> MALRAMRGIVNGAAPELPVPTSGPLAGSREQALAVSRNYLSQPRLTYKTVSGVNGPLVILDHVKFPRYAEIVHLTLPDGTKRSGQVLEVSGSKAVVQVFEGTSGIDAKKTSCEFTGDILRTPVSEDMLGRVFNGSGKPIDRGPVVLAEDFLDIMGQPINPQCRIYPEEMIQTGISAIDGMNSIARGQKIPIFSAAGLPHNEIAAQICRQAGLVKKSKDVVDYSEENFAIVFAAMGVNMETARFFKSDFEENGSMDNVCLFLNLANDPTIERIITPRLALTTAEFLAYQCEKHVLVILTDMSSYAEALREVSAAREEVPGRRGFPGYMYTDLATIYERAGRVEGRNGSITQIPILTMPNDDITHPIPDLTGYITEGQIYVDRQLHNRQIYPPINVLPSLSRLMKSAIGEGMTRKDHADVSNQLYACYAIGKDVQAMKAVVGEEALTSDDLLYLEFLQKFER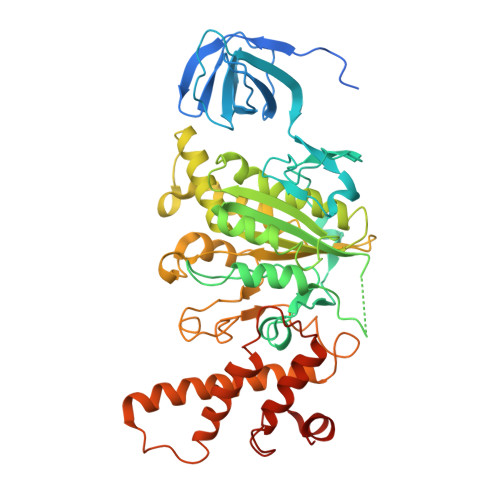NFIAQGPYENRTVYETLDIGWQLLRIFPKEMLKRIPQSTLSEFYPRDSAKH Aerolysin is a major contributor to the pathogenicity of Aeromonas spp, which causes gastroenteritis, deep wound infections and sepsis in humans. It is a pore-forming toxin (PFT), which is secreted by the bacterium as a water-soluble protein, binds receptors on their target cell membrane and, following proteolytic activation, forms circular heptameric oligomers that insert into the plasma membrane thus permeabilizing it, potentially leading to cell death. Aerolysin belongs to the family of β-PFTs, meaning that the final pore spans the membrane in the form of a β-barrel and defines the aerolysin-like family of proteins that share a common structural motif3. Combined, these structures, consistent with the recent lysenin pore structure, describe the major steps involved in the pore-formation process by aerolysin: the transition from the monomer to the oligomer with the formation of two highly stable concentric β-barrels, the zipper-like formation of the β-barrel and the final piston-like puncturing of the lipid bilayer.

While the wild-type aerolysin pore is a membrane-inserted heptamer, a single-point mutant Y221G was found to arrest the protein in its prepore stage. The cryo-EM map of Y221G, shown previously to be a head-to-head dimer of heptamers in solution was here determined at a global resolution of 3.9 Å, extending to 3.0–3.5 Å in most parts of the complex, allowing most bulky side chains to be resolved. Domain 1, which is connected to domain 2 by a long amino-acid stretch, rotates by 180° and moves by 30 Å. Following this movement, all receptor-binding sites become ideally located with respect to the target membrane (D1, D2 and dashed line in Fig. 1c,d). Domains 2 and 3 are mostly unchanged with respect to the soluble structure (1.3 and 3.4 Å root mean squared deviations, respectively). In particular, the prestem loop remains locked in the same curled-up position (yellow loop in Fig. 1e). Upon CTP removal, the β-strands rearrange to form a β-sandwich in the core of which the hydrophobic residues are buried. Furthermore, domain 4 straightens with respect to domain 3 and moves by 20 Å (turquoise domain in Fig. 1e). The high-resolution aerolysin prepore structure, thus reveals an elegant novel fold consisting of two concentric β-barrels held together by interaction of hydrophobic side chains.

>[14x]AEPVYPDQLRLFSLGQGVCGDKYRPVNREEAQSVKSNIVGMMGQWQISGLANGWVIMGPGYNGEIKPGTASNTWCYPTNPVTGEIPTLSALDIPDGDEVDVQWRLVHDSANFIKPTSYLAHYLGYAWVGGNHSQYVGEDMDVTRDGDGWVIRGNNDGGCDGYRCGDKTAIKVSNFAYNLDPDSFKHGDVTQSDRQLVKTVVGWAVNDSDTPQSGYDVTLRGDTATNWSKTNTYGLSEKVTTKNKFKWPLVGETELSIEIAANQSWASQNGGSTTTSLSQSVRPTVPARSKIPVKIELYKADISYPYEFKADVSYDLTLSGFLRWGGNAWYTHPDNRPNWNHTFVIGPYKDKASSIRYQWDKRYIPGEVKWWDWNWTIQQNGLSTMQNNLARVLRPVRAGITGDFSAESQFAGNIEIGAPVPLAA>[4x]MKGYTVPLSPRGIANLAPAPPWHYAGTVVGVEFFTDPAAAAATLPEGLTPDPDSAGRGVAMFIDWQYSSTGLEYLDPARSQYREFLITLDAHCNGAPVAWCPYIYVDNDAAMARGWVQGFPKKLGAVHQTRAYSVGGPGTPVLGPGGQFGATASSAGQRIAEAKITLEQPVPDPAALMSRPVINLRHFPRLAAGQHDQPAVHELVMSVLDDTAVSDAWVGTADLAFLPAHG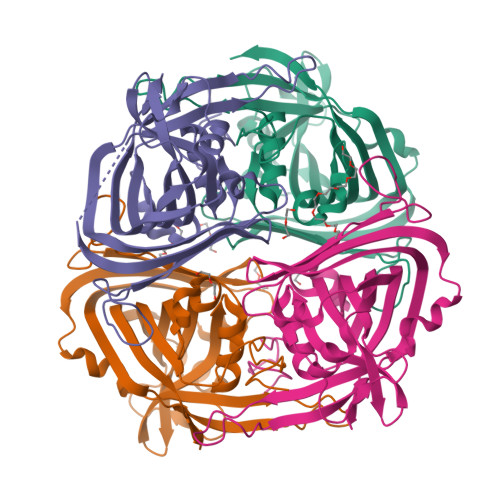EELADLPVRRTGKGFHFDLAYTVTDLMTLADHSA>MTQGAVKTTGKRSRAVSAKKKAILSAALDTFSQFGFHGTRLEQIAELAGVSKTNLLYYFPSKEALYIAVLRQILDIWLAPLKAFREDFAPLAAIKEYIRLKLEVSRDYPQASRLFCMEMLAGAPLLMDELTGDLKALIDEKSALIAGWVKSGKLAPIDPQHLIFMIAASTQHYADFAPQVEAVTGAT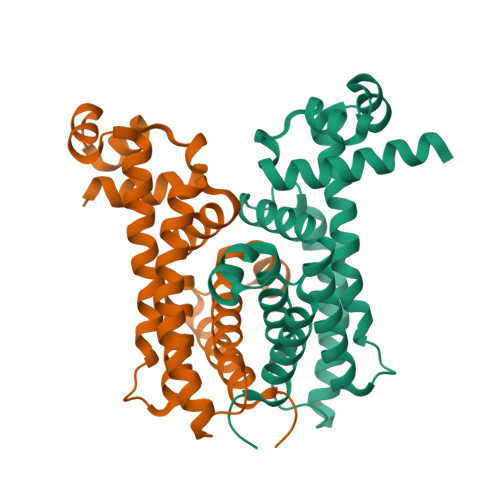LRDEVFFNQTVENVQRIIIEGIRPRLGHHHHHH[2x]>[2x]MRSNSVNIETFKDMLKRYEDFKMKNKREPRVIFIRSGGGESIPLETFRDMVRRYNNFKDRYGREPRIVYVTPPEPPVPEVNENTPEYVSITQFKDMLSRYNRFKEVNGREPRVVFIYSGGGPSVSLETFKDMCKRYNQFLEENRREPRIVYVTPPEPPVPEEVREMRRVLGEFKTATQLYTLVSRRCKYKFYYNDQTPNREALKKMVTDGINCTDACQLFKPVIEGLGYSVRIEHVKVRCN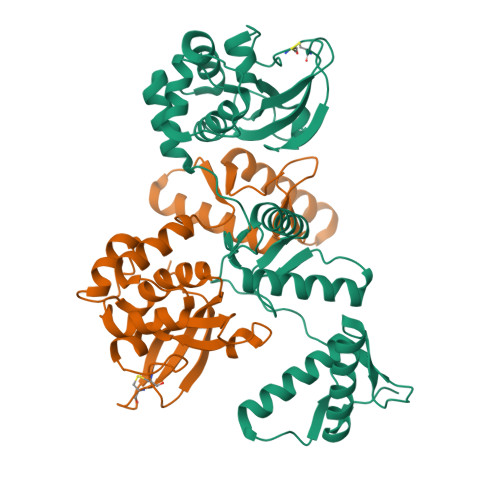DNKWYGHYFLRVAGKELASVSLPSERWTVWDYVSATKTGRPLGAPCCSRGIQHLGWGIVSPK>[2x]EAIRYSIPE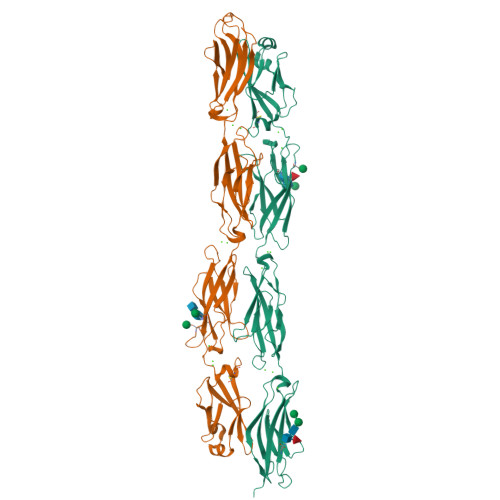ETESGYLVAHLAKDLGFRVGELATRRARIHHRGNKELLQLDVETGNLLLKEKPDREALCGATEPCVLHFQIILENPVQFFQTELQLTDINDHSPEFPDTEMLLKIQESTQPATVFLLKAAQDSDIGSNAVQNYTVSPNLHFHVVTLSRSDGRKYPELVLDRALDREEQPELTLILTALDGGAPPKSGTTTVRIEVVDINDNAPEFVQSLYSVEVPENSPLDALVVTVSARDLDAGIHGNVAYSLFQGGGGPQPFVIDEITGEIRLKGALDFEATSYYTMEIVATDSGGLSGKCTVAIQVLDVNDNAPKLTISSLTSSIPENAPEAVVAVFSVSDPDSGDNGRMVCSIQNELPFLLKPTFENYYTLAAEGPLDREIREEYNITIIVSDLGTPRLTTQHTITVQVVDINDHHHHHHHH> MGRVRLVQFQKNTDEPMGITLKMNELNHCIVARI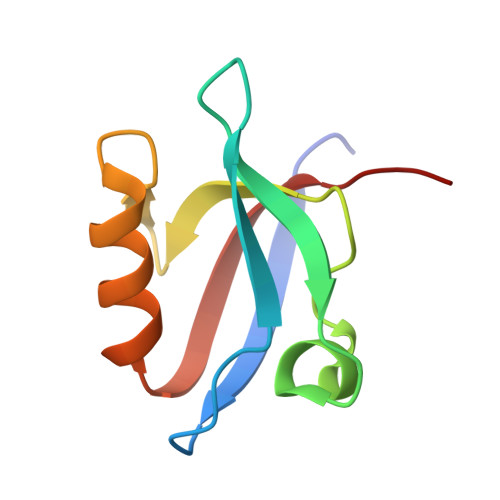MHGGMIHRQGTLHVGDEIREINGISVANQTVEQLQKMLREMRGSITFKIVPSYR>MCGIWALFGSDDCLSVQCLSAMKIAHRGPDAFRFENVNGYTNCCFGFHRLAVVDPLFGMQPIRVKKYPYLWLCYNGEIYNHKKMQQHFEFEYQTKVDGEIILHLYDKGGIEQTICMLDGVFAFVLLDTANKKVFLGRDTYGVRPLFKAMTEDGFLAVCSEAKGLVTLKHSATPFLKVEPFLPGHYEVLDLKPNGKVASVEMVKYHHCRDVPLHALYDNVEKLFPGFEIETVKNNLRILFNNAVKKRLMTDRRIGCLLSGGLDSSLVAATLLKQLKEAQVQYPLQTFAIGMEDSPDLLAARKVADHIGSEHYEVLFNSEEGIQALDEVIFSLETYDITTVRASVGMYLISKYIRKNTDSVVIFSGEGSDELTQGYIYFHKAPSPEKAEEESERLLRELYLFDVLRADRTTAAHGLELRVPFLDHRFSSYYLSLPPEMRIPKNGIEKHLLRETFEDSNLIPKEILWRPKEAFSDGITSVKNSWFKILQEYVEHQVDDAMMANAAQKFPFNTPKTKEGYYYRQVFERHYPGRADWLSHYWMPKWINATDPSARTLTHYKSAVKA[2x]

Asparagine synthetase (ASNS) catalyzes the ATP-dependent biosynthesis of L-asparagine in cells from l-aspartic acid using l-glutamine as a nitrogen source. Several recent findings provide evidence for connections between asparagine biosynthesis and human disease, raising the urgency for in-depth studies of human ASNS. As seen for the bacterial homolog, human ASNS is composed of two domains. Residues in the C-terminal (residues 203–560) synthetase domain (41.6% identity) are more conserved than those in the N-terminal (residues 1–202) glutaminase domain (33.9% identity) based on sequence comparisons of human ASNS and its homologs in a number of model organisms.

In order to determine the molecular basis for the binding selectivity of ASNS inhibitor 1 and to provide a firm basis for future, structure-based efforts to identify potent and selective ASNS inhibitors with simplified molecular scaffolds, we determined the high-resolution crystal structure of human ASNS by X-ray crystallography at 1.85 Å resolution. Conditions were then identified that gave a single crystal of the DON-modified enzyme, which diffracted to 1.85 Å resolution. Two molecules of DON-modified human ASNS were present in the asymmetric unit as a head-to-head dimer in which the two monomers were linked by a disulfide bond that likely forms during crystallization. A cis-proline (Pro-60) linkage is present in the human enzyme identical to that in the structure of the bacterial homolog AS-B. Electron density for the DON-modified Cys-1 side chain is clearly evident in each monomer. A hydrogen bond network, composed of the conserved residues Arg-48, Val-52, Asn-74, Gly-75, Glu-76, and Asp-96, which mediates substrate recognition and thioester stabilization in the hydrolysis reaction that produces ammonia, is also clearly defined. This substrate-binding pocket is located at the interface of the two domains and is within 5 Å of an absolutely conserved glutamate residue (Glu-414) in the C-terminal domain. After refinement of the protein and ligands, a single 12 σ peak remained in a pocket at the interface of the N- and C-terminal domains on both chains. The site is surrounded by Tyr-78, Arg-416, Arg-245, and Val-417, and the peak was assigned as a chloride anion. Importantly for structure-based inhibitor discovery, the synthetase site in the C-terminal domain, which is composed of sixteen α-helices and five β-strands, is well resolved. We also observed density consistent with a bound HEPES molecule from the crystallization buffer in this domain, which hydrogen bonds to the Asp-334 side chain and water molecules in a network that also involves conserved residues Asp-400 and Arg-403.>[2x]MFERIDYYAGDPILGLVEKFAADNNPDKVNLGIGIYYDESGVMPVLDCVKIAEQRIADPISPRPYLPMAGLPGHRKGCQELLFGKDAPVLKDGLVATIATIGGSGALKVGAEFIHEWFPQSKCYVSDPTWGNHIAIFEGCDIEVGKYPYYDTATGGIKFDEMIAFFETLNKDD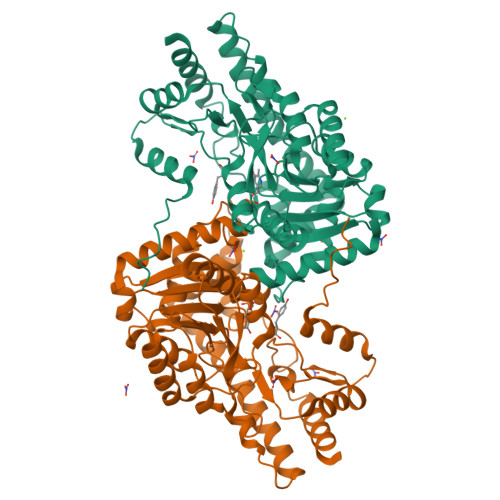VLLLHPCCHNPTGVDLTREQWDTVLNVIQERELIPFMDIAYQGFGEDMDSDAYAIRKAVDMGLPLFVSNSFSKNLSLYGERVGGLSVVCPTVDETERVFGQLNSTVRRIYSSPPSHGGRVVDIVMNDAALHEQWVGEVYAMRDRIKSMRTKLKSVLEAKISGRNFDYLTAQNGMFSFTGLTPEQVERLQSEFGIYMISNSRMCVAGLNSSNIDYVANAMVDVLKD>MHHHHHHSAGENLYFQGKEWQENKSWNAHFTEHKSQGVVVLWNENKQQGFTNNLKRANQAFLPASTFKIPNSLIALDLGVVKDEHQVFKWDGQTRDIATWNRDHNLITAMKYSVVPVYQEFARQIGEARMSKMLHAFDYGNEDISGNVDSFWLDGGIRISATEQISFLRKLYHNKLHVSAASQRIVKQAMLTEANGDYIIAAKTGYSTRIEPKIGWWVGWVELDDNVWFFAMNMDMPTSDGLGLRQAITK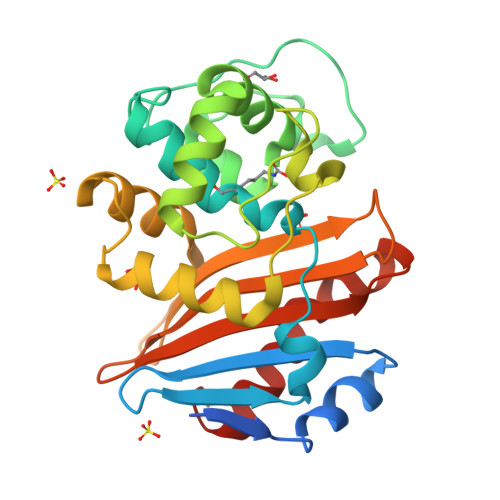EVLKQEKIIP[2x]>[2x]MDHLPIFCQLRDRDCLIVGGGDVAERKARLLLEAGARLTVNALTFIPQFTVWANEGM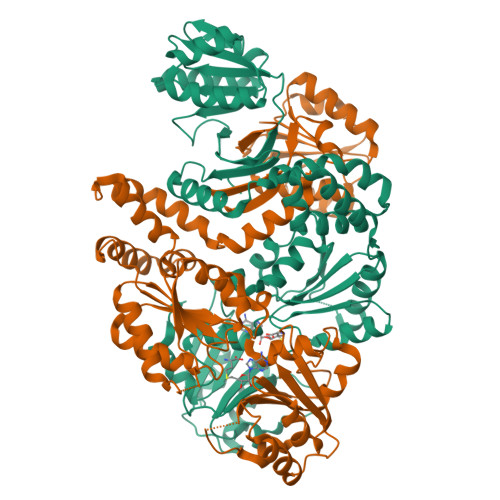LTLVEGPFDETLLDSCWLAIAATDDDTVNQRVSDAAESRRIFCNVVDAPKAASFIMPSIIDRSPLMVAVSAGGTSPVLARLLREKLESLLPQHLGQVARYAGQLRARVKKQFATMGERRRFWEKFFVNDRLAQSLANADEKAVNATTERLFSEPLDHRGEVVLVGAGPGDAGLLTLKGLQQIQQADIVVYDRLVSDDIMNLVRRNADRVFVGKRAGYHCVPQEEINQILLREAQKGKRVVRLKGGDPFIFGRGGEELETLCHAGIPFSVVPGITAASGCSAYSGIPLTHRDYAQSVRLVTGHLKTGGELDWENLAAEKQTLVFYMGLNQAATIQEKLIAFGMQADMPVALVENGTSVKQRVVHGVLTQLGELAQQVESPALIIVGRVVALRDKLNWFSNH> MEILEEKPKEGKVKVKAETLDDLWHLYHIIDPGDIVYAKTLRKQAQRADSLRAEKVEVIPVFLGVQAEKINF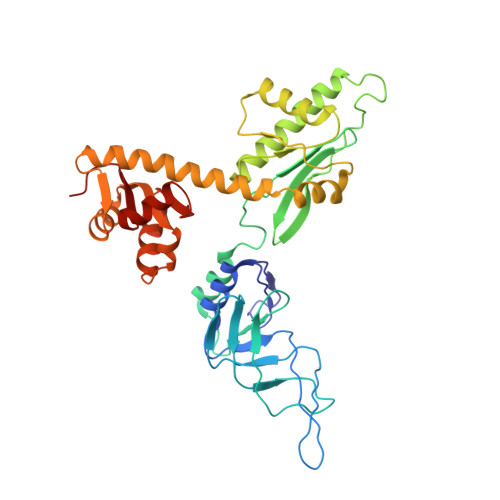HKFANQVRVTGPIVYASREDVPLGKYHTIAIEQGTVVTIQKPRWKEHHIERLKEAVAASKRARVMIVVIDDGEADMALVREYGVEILNSIRHNLGGKRYNTDRESEEMKFFHDVAKTMEEVMKRENVEKAIVAGPGFVKEDFYKFLKEKYPELAKKVVIEDTSVTGRTGIYEVIKRGVVDRVYQENRVAKEVQLVEKVLENIARNNGLVAYGLKEVEEAVNYGAVETLLVLDELLKGELREKVEELMDAVRYSRGEVVVVSSEHEGGEKLKALGGLAALLRFRVK>TETTSFLITKFSPDQQNLIFQGDGYTTKEKLTLTKAVKNTVGRALYSSPIHIWDRETGNVANFVTSFTFVINAPNSYNVADGFTFFIAPVDTKPQTGGGYLGVFNSAEYDKTTQTVAVEFDTFYNAAWDPSNRDRHIGIDVNSIKSVNTKSWKLQNGEEANVVIAFN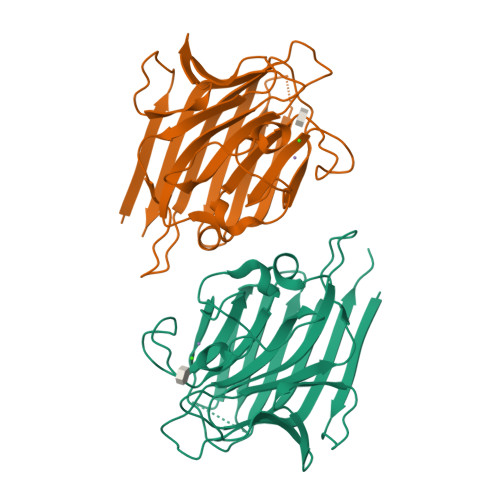AATNVLTVSLTYPNSLEEENVTSYTLSDVVSLKDVVPEWVRIGFSATTGAEYAAHEVLSWSFHSELSGT[2x]>SNAMIRDTATNTTQTQAAPQQAPAQQFTQAPQEKPMQSTQSQPTPSYAGTGGINSQFTRSGNVQGGDARASEALTVFTRLKEQAVAQQDLADDFSILRFDRDQHQVGWSSLVIAKQISLNGQPVIAVRPLILPNNSIELPKRKTNIVNGMQTDVIESDIDVGTVFSAQYFNRLSTYVQNTLGKPGAKVVLAGPFPIPADLVLKDSELQLRNLLIKSVNACDDILALHSGERPFTIAGLKGQQGETLAAKVDIRTQPLHDTVGNPIRADIVVTTQRVRRNGQQENEFYETDVKLNQVAMFTNLERTPQAQAQTLFPNQQQVATPAPWVASVVITDVRNADGIQANTPEMYWFALSNAFRSTHGHAWARPFLPMTGVAKDMKDIGALGWMSALRNRIDTKAANFDDAQFGQLMLSQVQPNPVFQIDLNRMGETAQMDSLQLDAAGGP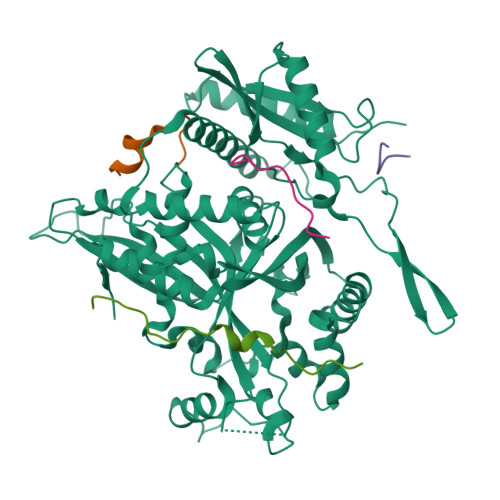NAQKAAATIIRQINNLGGGGFERFFDHTTQPILERTGQVIDLGNWFDGDEKRDRRDLDNLAALNAAEGNENEFWGFYGAQLNPNLHPDLRNRQSRNYDRQYLGSTVTYTGKAERCTYNAKFIEALDRYLAEAGLQITMDNTSVLNSGQRFMGNSVIGNNMVSGQAQVHSAYAGTQGFNTQYQTGPSSFY[5x]(3S)-3,4-dimethyl-3-propyl-3,4-dihydro-1H-1,4-benzodiazepine-2,5-dione | C14 H18 N2 O2 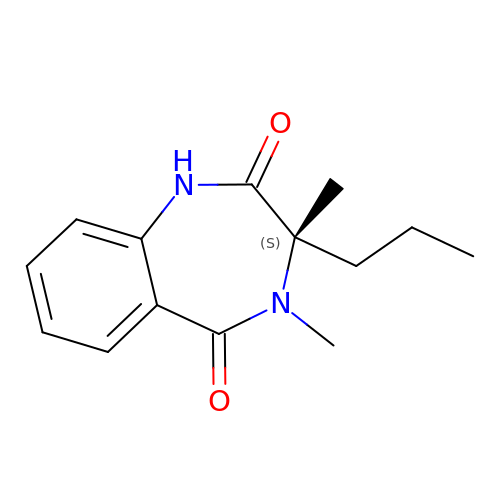| CNQOZARVGPMUHF-AWEZNQCLSA-N4-(4-nitrobenzyl)pyridine 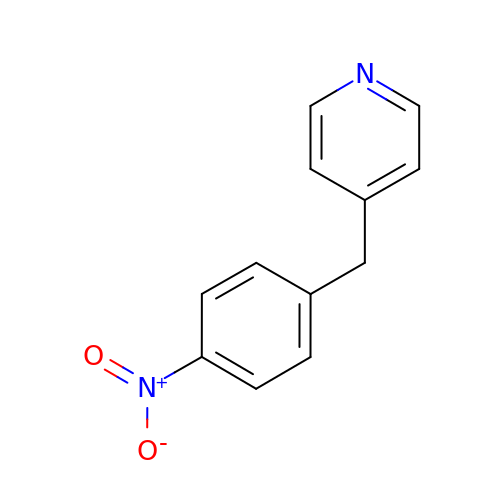| C12 H10 N2 O2 | MNHKUCBXXMFQDM-UHFFFAOYSA-N>[2x]SNA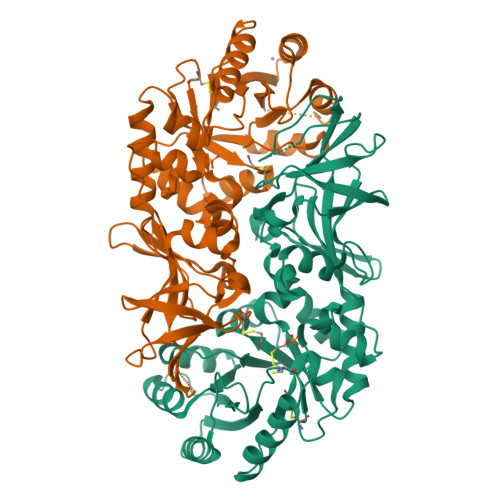MSDKYYRSAYMNVDLNAVASNFKVFSTLHPNKTVMAVVKANAYGLGSVKVARHLMENGATFFAVATLDEAIELRMHGITAKILVLGVLPAKDIDKAIQHRVALTVPSKQWLKEAIKNISGEQEKKLWLHIKLDTGMGRLGIKDTKTYQEVIEIIQQYEQLVFEGVFTHFACADEPGDMTTEQYQRFKDMVNEAIKPEYIHCQNSAGSLLMDCQFCNAIRPGISLYGYYPSEYVQQKVKVHLKPSVQLIANVVQTKTLQAGESVSYGATYTATDPTTIALLPIGYADGYLRIMQGSFVNVNGHQCEVIGRVCMDQTIVKVPDQVKAGDSVILIDNHRESPQSVEVVAEKQHTINYEVLCNLSRRLPRIYHDGDQRFVTNELLK>[2x]KLATDIENNVRVVVYIRKDVEDNSQTIEKEGQTVTNNDYHKVYDSLKNMSTVKSVTFSSKEEQYEKLTEIMGDNWKIFEGDANPLYDAYIVEANAPNDVKTIAEDAKKIEGVSEVQD

FtsEX comprises a cell division-regulating integral membrane protein (FtsX) and a cytoplasmic ATPase (FtsE) that resembles an ATP-binding cassette (ABC) transporter. Hydrolysis causes a conformational change that is transmitted through the membrane via FtsX, an integral membrane protein with two extracellular loops (ECLs), denoted the large (ECL1) and small (ECL2) loops. The folded structure (residues 57 to 166) reveals a central core composed of a four-stranded antiparallel β-sheet (β1, β6, β4, and β5) and two helices (α1 and α3), an α-helical lobe (residues 107 to 135) harboring the α2 helix, and an extended β-hairpin (β2 and β3). The helical lobe mediates a physical interaction with the peptidoglycan hydrolase PcsB via the coiled-coil domain of PcsB (PscBCC).

Three different structures, with resolutions ranging from 2.0 to 2.3 Å, were solved by X-ray crystallography, each in the presence of a different detergent. The detergents used were dodecyltrimethylammonium chloride (detergent 1 [D1]), n-undecyl-β-d-maltoside (detergent 2 [D2]), and n-decyl-β-d-maltoside (detergent 3 [D3]). In all cases, two independent protein molecules are present in the asymmetric unit, arranged in such a way as to keep hydrophobic residues from their α-helical lobes buried. Different conformations were observed for the β-hairpin and the helical lobe among the six structures, depending on the presence and identity of the detergent molecule bound to FtsXECL1. In any case, the crystal structures suggest that changes in the protein backbone and side chains of the helical lobe occur when a detergent ligand is bound. These changes create a cavity in which the detergent molecules insert, with a large part of the helical lobe (from Q111 to E127) affected by the interaction with detergent. Residues Y112, W123, E127, and F126 are strongly perturbed upon detergent ligand binding, with the hydroxyl moiety of Y112 interacting with carboxylate of E127. Changes in W123 and F126 stabilize the hydrophobic region of detergent 1. A similar interaction pattern is observed for detergents 2 and 3; additional interactions are observed in N131 with detergents 2 and 3, which are characterized by a larger hydrophilic head (maltose). Full stabilization of the hydrophobic tail of the detergents is completed by the same hydrophobic residues (W123 and F126) but from a symmetry-related molecule.>PCQNHHCKHGKVCELDENNTPMCVCQDPTSCPAPIGEFEKVCSNDNKTFDSSCHFFATKCTLEGTKKGHKLHLDYIGPCKYIPPCLDSELTEFPLRMRDWLKNVLVTLYERDEDNNLLTEKQKLRVKKIHENEKRLEAGDHP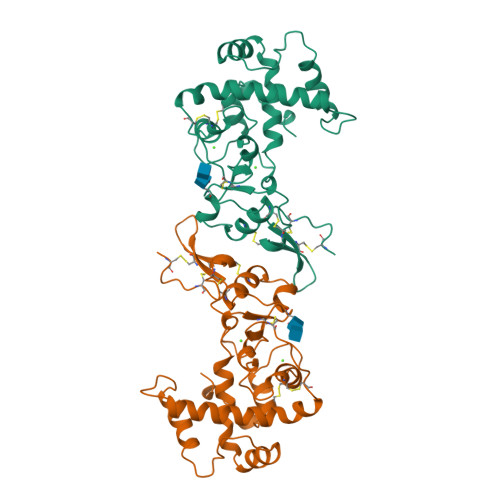VELLARDFEKNYNMYIFPVHWQFGQLDQHPIDGYLSHTELAPLRAPLIPMEHCTTRFFETCDLDNDKYIALDEWAGCFGIKQKDIDKDLVI[2x]>[2x]MEVKIFNTQDVQDFLRVASGLEQEGGNPRVKQIIHRVLSDLYKAIEDLNITSDEYWAGVAYLNQLGANQEAGLLSPGLGFDHYLDMRMDAEDAALGIENATPRTIEGPLYVAGAPESVGYARMDDGSDPNGHTLILHGTIFDADGKPLPNAKVEIWHANTKGFYSHFDPTGEQQAFNMRRSIITDENGQYRVRTILPAGYGCPPEGPTQQLLNQLGRHGNRPAHIHYFVSADGHRKLTTQINVAGDP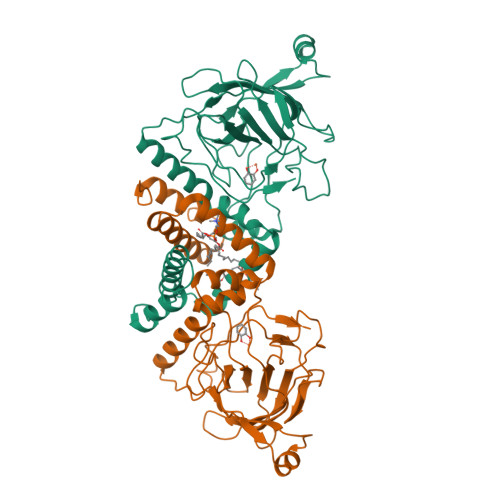YTYDDFAYATREGLVVDAVEHTDPEAIKANDVEGPFAEMVFDLKLTRLVDGVDNQVVDRPRLAV>[8x]SMTVPSNTPYSGEYGFEISFQHQSKETKSTTWTFSESLKKLFVRMATTCPVRFKTVHQPPAGSVIRAMPIYVKPEHVQEVVKRCPNHATTKEHNEDHPAPTHLVRCEHKLASYVEDPYTGRQSVIIPQEHPQAGAEWVTNLYQFMCFSSCVGGLNRRPIQVIFTLEHEGVVLGRQAVEVRICACPGRDRRAEETAADPNKQQKR

Low intrinsic stability is a crucial factor for the susceptibility of the transcription factor p53 to inactivating mutations in human cancer. To gain further insights into the evolutionary history of p53 and factors that govern the stability of p53 family proteins, we have characterized the DBD of a p53 homolog from the extremophilic annelid Alvinella pompejana, which lives in tubes at the edge of hydrothermal vents at the bottom of the Pacific. We show that it has a p53/p63-like DBD that is more thermostable than all vertebrate p53 DBDs tested so far, but, intriguingly, not as stable as human p63. In addition, the A. pompejana homolog shares DNA-binding properties with human p53 family DBDs, despite its evolutionary distance, consistent with a potential role in maintaining genome integrity.

We determined the crystal structure of the A. pompejana DBD at 1.92 Å resolution. The overall structure consists of an immunoglobulin-like β-sandwich, which serves as a scaffold for an extended DNA-binding surface. The latter is formed by a loop-sheet-helix motif and two large loops that are held together by zinc coordination. The zinc-binding site (Cys176, His179, Cys238, and Cys242) is conserved in A. pompejana. Key DNA-contact residues are also conserved: Arg248 in Loop L3 for minor groove binding, Arg273, which interacts with the phosphate backbone, and Arg280 in the C-terminal helix that interacts with guanine in the major groove in human p53-DNA complexes. Structural differences were found mainly on the surface and in loop regions, for example in the L1 loop, which plays a unique role in DNA recognition by human p53. In A. pompejana, there is much less divergence in this loop, apart from a one-residue insertion at its N-terminal base. However, the overall conformation differs significantly from that seen in human p53, adopting a much more recessed orientation, with a high degree of disorder observed in most chains of the asymmetric unit. Intriguingly, A. pompejana has a similar large-to-small substitution at this position, F270V, but in this case, the crystal structure of the DBD shows that the substitution is compensated for by a small-to-large substitution of a neighboring residue, I255F, which maintains optimal packing of the hydrophobic core. The additional tryptophan-mediated hydrophobic packing interactions are likely to contribute to the increased thermostability of the A. pompejana DBD, and also that of the p63/p73 DBD, which is supported by mutagenesis studies on human p53.>[2x]RLPDAPTLKRMTARFAPVDVKVDVSKLPDAEKRALAKILQAAKIMDPLFLSQAWAGNPTLLLDLVEDTTPLGKERLHAFLLNKGPWSRLDEAKPFIPGVPPKPDEGNFYPAGATKAEVEAWVKSLPEAQQHAATGFFTTVRKGPDGKFLTVPYSVEYQGELGMAAKLLREAAALTQQSTLKRFLETRAEAFLSNDYYASEVAWMELDASVEPTIGPYEVYEDGWFNYKAAFEAFIGVRDEAETQKLAKFSAELQELENNLPIEPALRNPKLGALAPIRVINSLYSSGDGNRGVQTAAYNLPNDERVAAEKGTKRVMLKNIQ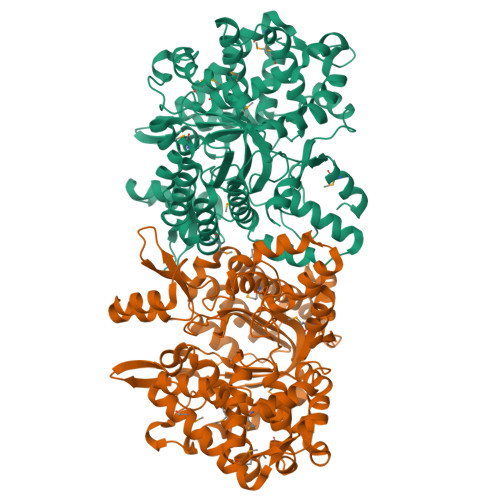EAKFQRVLVPIAKVALPAKDRKDVSFDAFFTHILMHELMHGLGPHNVTVAGKQTTVRQALQASSSAIEEAKADISGLWALQRLVDKGTLDKELQRTMYTTFLASAFRSIRFGIDEAHGKGIALQLNHFLDTGAVKVNADGTFEVVPDKMQASVTSLTNQLMSLQAKGDRAAAEELLAKQGVVRPSVQKVLEKLKNVPVDIEPRYVTAESLVKDFGA> GPHMRKSQQAEREYEKIKSQLEGLEESVRDRCKKEFTDLMIEMEDQTNDVHEAGIPTLDYKTYTDRVFFLPSKDGDKDVMITGKLDIPESRRPIVEQA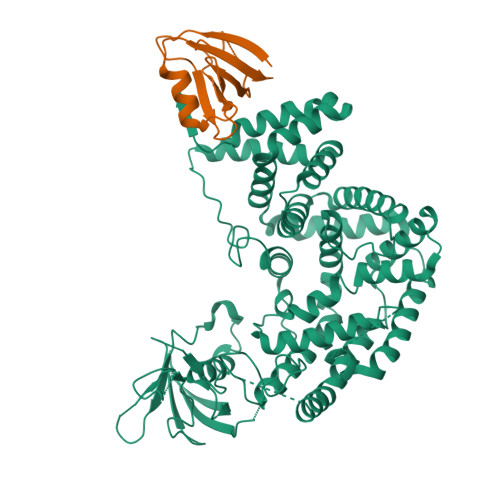LYQFSNLLNSKSFLINFIHTLENQREFSARAKVYFASLLTVALHGKLEYYTDIMRTLFLELMEQYVVAKNPKLMLRRSETVVERMLSNWMSICLYQYLKDSAGEPLYKLFKAIKHQVEKGPVDAVQKKAKYTLNDTGLLGDDVEYAPLTVSVIVQDEGIDAIPVKVLNCDTISQVKEKIIDQVYRTQPCSCWPKPDSVVLEWRPGSTAQILSDLDLTSQREGRWKRINTLMHYNVRDGATLILSKVGVSQQPEDSQQDLPGERHALLEEENRVWHLVRPTDEVDEGKSKRGSMKEKERTKAITEIYLTRLLSVKGTLQQFVDNFFQSVLAPGHAVPPAVKYFFDFLDEQAEKHDIRDEDTIHIWKTNSLPLRFWVNILKNPHFIFDVHVHEVVDASLSVIAQTFMDACTRTEHKLSRDSPSNKLLYAKEISTYKKMVEDYYKGIRQMVQVSDQDMNTHLAEISRAHTDSLNTLVALHQLYQYTQKYYDEIINALEEDPAAQKMQLAFRLQQIAAALENKVTDL;> GPHMGLVQRCVIIQKDQHGFGFTVSGDRIVLVQSVRPGGAAMKAGVKEGDRIIKVNGTMVTNSSHLEVVKLIKSGAYVALTLLGSSPS> MAMITGGELVVRTLIKAGVEHLFGLHGAHIDTIFQACLDHDVPIIDTRHEAAAGHAAEGYARAGAKLGVALVTAGGGFTNAVTPIANAWLDRTPVLFLTGSGALRDDETNTLQAGIDQVAMAAPITKWAHRVMATEHIPRLVMQAIRAALSAPRGPVLLDLPWDILMNQIDEDSVIIPDLVLSAHGARPDPADLDQALALLRKAERPVIVLGSEASRTARKTALSAFVAATGVPVFADYEGLSMLSGLPDAMRGGLVQNLYSFAKADAAPDLVLMLGARFGLNTGHGSGQLIPHSAQVIQVDPDACELGRLQGIALGIVADVGGTIEALAQATAQDAAWPDRGDWCAKVTDLAQERYASIAAKSSSEHALHPFHASQVIAKHVDAGVTVVAD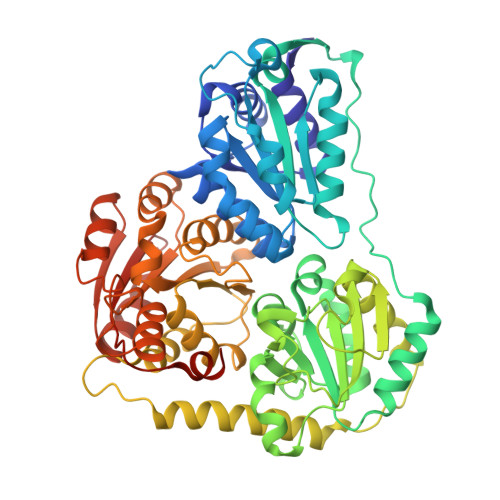GALTYLWLSEVMSRVKPGGFLCHGYLGSMGVGFGTALGAQVADLEAGRRTILVTGDGSVGYSIGEFDTLVRKQLPLIVIIMNNQSWGATLHFQQLAVGPNRVTGTRLENGSYHGVAAAFGADGYHVDSVESFSAALAQALAHNRPACINVAVALDPIPPEELIIIGMDPFA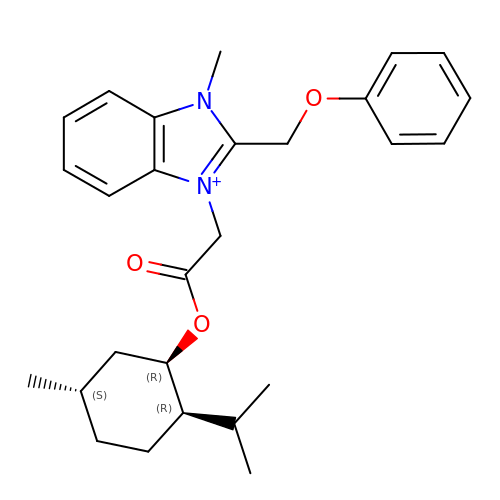1-methyl-3-(2-{[(1R,2R,5S)-5-methyl-2-(propan-2-yl)cyclohexyl]oxy}-2-oxoethyl)-2-(phenoxymethyl)-1H-1,3-benzimidazol-3-ium | C27 H35 N2 O3 | HACNGQQLOZYIEB-NIRIFSCTSA-N4-[[4-[4-(imidazolidin-2-ylideneamino)phenyl]-1,2,3-triazol-1-yl]methyl]benzohydrazide 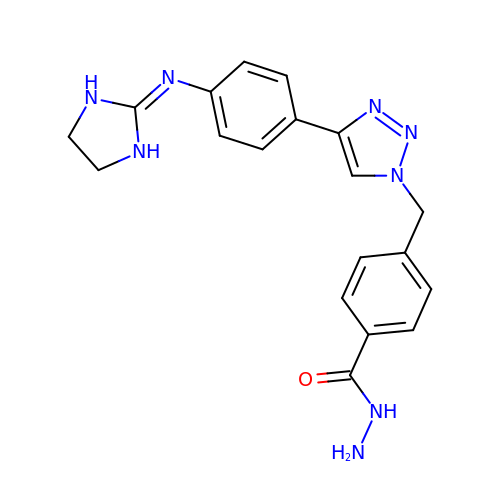| C19 H20 N8 O | FNWSHZHKFUFPQJ-UHFFFAOYSA-N> MDDKELIEYFKSQMKEDPDMASAVAAIRTLLEFLKRDKGETIQGLRANLTSAIETLCGVDSSVAVSSGGELFLRFISLASLEYSDYSKCKKIMIERGELFLRRISLSRNKIADLCHTFIKDGATILTHAYSRVVLRVLEAAVAAKKRFSVYVTESQPDLSGKKMAKALCHLNVPVTVVLDAAV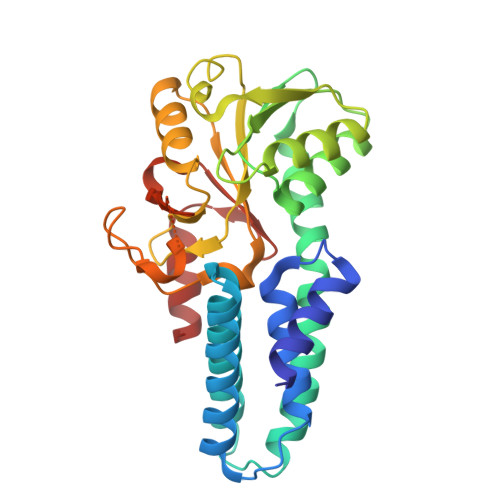GYIMEKADLVIVGAEGVVENGGIINKIGTNQMAVCAKAQNKPFYVVAESFKFVRLFPLNQQDVPDKFKYKADTLKVAQTGQDLKEEHPWVDYTAPSLITLLFTDLGVLTPSAVSDELIKLYL>HHHHVKLSVVEQAPVVEGLTPAHSLQHSIELARLADRLGYERFWVAEHHAEIFNAVPAPEILIARIAAETSGIRVGSGGVLLSLYSPLKVAEVFRTLHALYPDRIDLGIGRANRVKLPVFAALRDDTAGKEPSSDDLWRRLEQLRAYLDPDSGLPFTVSPRMPGGPALWLLGASVSSAEAAARLGLPYAYAHFITPQFTREAMDTYRAAFVPGPDTPSPRPILSVVVCCAETDAEAQRVYATHRLFHRRMSQGDVRLLPPADLAVAEMDKPGPD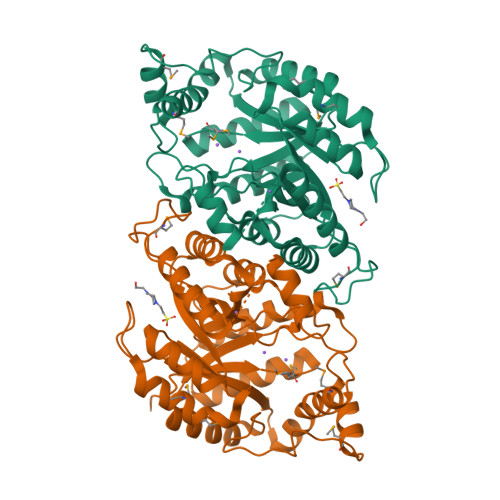PLAEESFEWPRYVVGSPDRVRDQLTKMADATGAEELGVVSMIHDQRDRLRSYRLLAEAFELTPR[3x];> HHHHVKLSVVEQAPVVEGLTPAHSLQHSIELARLADRLGYERFWVAEHHAEIFNAVPAPEILIARIAAETSGIRVGSGGVLLSLYSPLKVAEVFRTLHALYPDRIDLGIGRANRVKLPVFAALRDDTAGKEPSSDDLWRRLEQLRAYLDPDSGLPFTVSPRMPGGPALWLLGASVSSADAAARLGLPYAYAHFITPDFTREAMDTYRAAFVPGPDTPSPRPILSVVVCCAETDAEAQRVYATHRLFHRRMSQGDVRLLPPADLAVAEMDKPGPDPLAEESFEWPRYVVGSPDRVRDQLTKMADATGAEELGVVSMIHDQRDRLRSYRLLAEAFELTPR>MKFSNITIKNFRNFEKVNINLDNKNVIFGMNDIGKTNFLYALRFLLDKEIRKFGFNKSDYHKHDTSKKIEIILTLDLSNYEKDEDTKKLISVVKGARTSANADVFYIALESKYDDKELYGNIILKWGSELDNLIDIPGRGNINALDNVFKVIYINPLVDLDKLFAQNKKYIFEESQGNESDEGILNNIKSLTDQVNQQIGEMTIIKGFQQEITSEYRSLKKEEVSIELKSEMAIKGFFSDIIPYIKKDGDSNYYPTSGDGRRKMLSYSIYNYLAKKKYEDKIVIYLIEEPEISLHRSMQIALSKQLFEQSTYKYFFLSTHSPELLYEMDNTRLIRVHSTEKVVCSSHMYNVEEAYGSV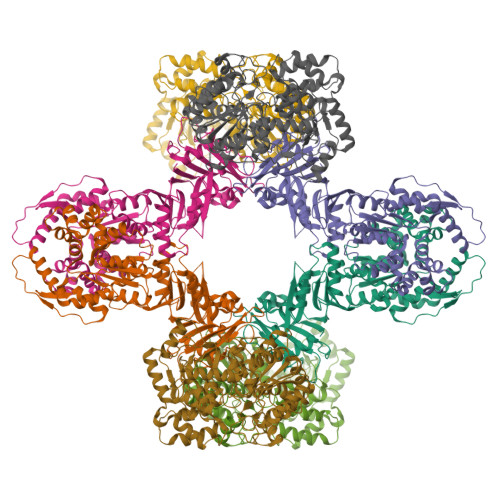KKKLNKALSSALFAERVLLIEGPSEKILFEKVLDEVEPEYELNGGFLLEVGGTYFNHYVCTLNDLGITHIIKTDNDLKSKKGKKGVYELLGLNRCLNLLGRENLDEITIDIPEDIKGKKKKERLNERKKEIFKQYKNEVGEFLGERIYLSEIDLENDLYSAIGESMKRIFENEDPVHYLQKSKLFNMVELVNNLSTKDCFDVFEHEKFACLKELVGSDRG[4x];>MIEDEMSREQIIKDGGNILVTAGAGSGKTTILVSKIEADLKENKTHYSIAAVTFTNKAAKEIEGRLGYSSRGNFIGTNDGFVESEIIRPFIKDAFGNDYPDNFTAEYFDNQFASYDKGLQVLKYQNILGTYSNPKKNFKFQLALDILKKSLVARQYIFSKYFKIFIDEYQDSDKDMHNLFMYLKDQLKIKLFIVGDPKQSIYIWRGAEPENFNGLIENSTDFNKYHLTSNFRCCQDIQNYSNLFNEETRSLIKEKNEVQNVISIADDMPISDILLKLTEEKQVLNIEAELVILVRRRNQAIEIMKELNEEGFNFIFIPQTPLDRATPNATLLKEVIKYVKNDRYSIYDLAAEIVGNLSSREIKEIQKIINELLVPNINQVLINQVLINLFAKLEITLDTREITAFTEVMMTNEFDIAFDTNEYLHKIFTVHSAKGLEFNQVIITASDYNVHYNRDTNEHYVATTRAKDKLIVIMDNKKYSDYIETLMKELKIKNIIKSI[4x]>[2x]AAAGKEKDVKVEVSVAVEELGTCSRSAIITVPASTVKDIFKRGVKRIERDVVGQLKGWQAGKPLPLSMVIQQVGGQNKFKTFCLEELLLEALPKGIESARNGRAVDPASVTVPPEDFPSMLERYDPA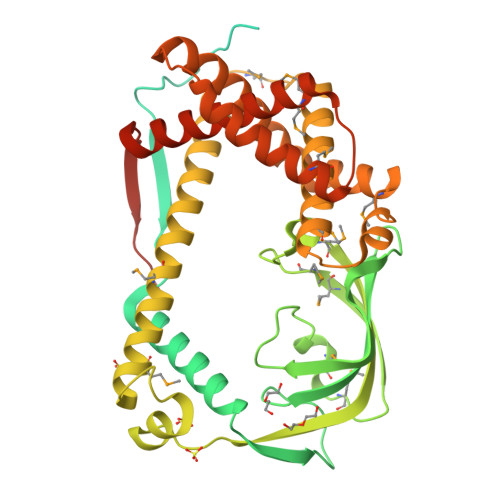KEFFFRAMFDVAPPVVWRTPLEELEVTIRDTGDFSTDAAAADDLIRQYRKQHGFSRVVAGRGLQLGDTLVIDLEITSKATGQALPGLTHKRFSFDTEADVLGITSGMLGMKAGESRTFNMSMPEDYDVEFWQSMPVKVAAKVHEIFEWTLPEFNDEYVAKQHEGKWGSAKEMREALIASTAMQRVTELDKALEDAVVKAVADALDMPEVPPRMVEQLGERQFQAQLLQMIEDRIGSREDVEKLATEEMAAEFIRERKKDLEDQVKFNLAVDDIWVRKGLVLEDEAVEAEFSLRARQMEAVGQPFDREDMLDDVRETVKSVTVIEWLKDNVKRHVLPYTAADDKAAKAKGEPVAV> GVENSGAGPTSFKTMKVIDPQHSDKPNVLILGSG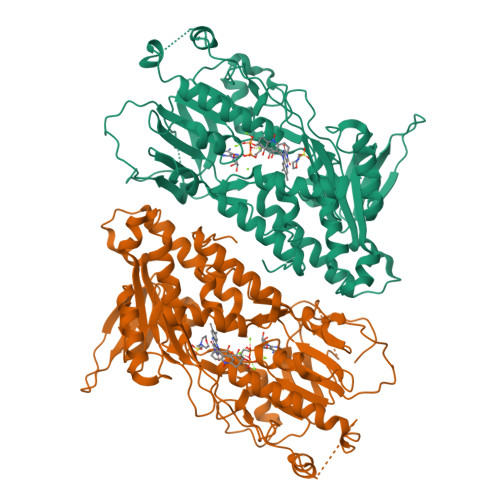WGAISFLKHIDTKKYNVSIISPRSYFLFTPLLPSAPVGTVDEKSIIEPIVNFALKKKGNVTYYEAEATSINPDRNTVTIKSLSAVSQLYQPENHLGLHQAEPAEIKYDYLISAVGAEPNTFGIPGVTDYGHFLKEIPNSLEIRRTFAANLEKANLLPKGDPERRRLLSIVVVGGGPTGVEAAGELQDYVHQDLRKFLPALAEEVQIHLVEALPIVLNMFEKKLSSYAQSHLENTSIKVHLRTAVAKVEEKQLLAKTKHEDGKITEETIPYGTLIWATGNKARPVITDLFKKIPEQNSSKRGLAVNDFLQVKGSNNIFAIGDNAFAGLPPTAQVAHQEAEYLAKNFDKMAQIPNFQKNLSSRKDKIDLLFEENNFKPFKYNDLGALAYLGSERAIATIRSGKRTFYTGGGLMTFYLWRILYLSMILSARSRLKVFFDWIKLAFFKRDFFKGL;> TGVENSGAGPTSFKTMKVIDPQHSDKPNVLILGSGWGAISFLKHIDTKKYNVSIISPRSYFLFTPLLPSAPVGTVDEKSIIEPIVNFALKKKGNVTYYEAEATSINPDRNTVTIKSLSAVSQLYQPENHLGLHQAEPAEIKYDYLISAVGAEPNTFGIPGVTDYGHFLKEIPNSLEIRRTFAANLEKANLLPKGDPERRRLLSIVVVGGGPTGVEAAGELQDYVHQDLRKFLPALAEEVQIHLVEALPIVLNMFEKKLSSYAQSHLENTSIKVHLRTAVAKVEEKQLLAKTKHEDGKITEETIPYGTLIWATGNKARPVITDLFKKIPEQNSSKRGLAVNDFLQVKGSNNIFAIGDNAFAGLPPTAQVAHQEAEYLAKNFDKMAQIPNFQKNLSSRKDKIDLLFEENNFKPFKYNDLGALAYLGSERAIATIRSGKRTFYTGGGLMTFYLWRILYLSMILSARSRLKVFFDWIKLAFFKRDFFKGL> MGSDKIHHHHHHVIVLGHRGYSAKYLENTLEAFMKAIEAGANGVELDVRLSKDGKVVVSHDEDLKRLFGLDVKIRDATVSELKELTDGKITTLKEVFENVSDDKIINIEIKEREAADAVLEISKKRKNLIFSSFDLD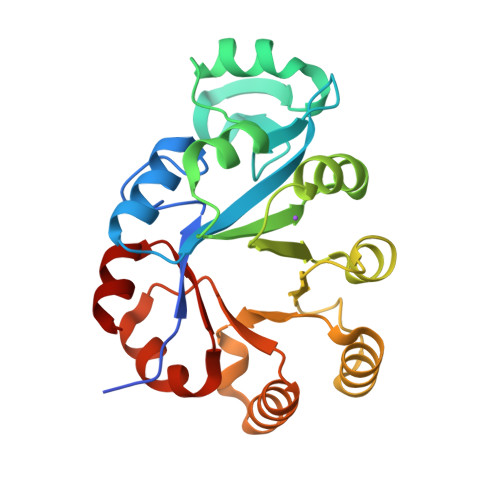LLDEKFKGTKYGYLIDEENYGSIENFVERVEKERPYSLHVPYQAFELEYAVEVLRSFRKKGIVIFVWTLNDPEIYRKIRREIDGVITDEVELFVKLR> SETDDLKWTERLPECPVYRPTKEEFEDPLTYLQKIFPEASKYGICKIVSPLTATVPAGAVLMKEKSNFKFTTRVQPLRLAEWDSDDKVTFFMSGRTYTFRDYEKMANKVFARRYCSGGSLPDSFLEKEFWKEIACGKTETVEYACDVDGSAFSSAPGDPLGSSKWNLNKVSRLPKSTLRLLETSIPGVTEPMLYIGMLFSMFAWHVEDHYLYSINYQHCGASKTWYGIPGSAALKFEKVVKECVYNDDILSTNGEDGAFDVLLGKTTIFPPKTLLDHNVPVYKAVQKPGEFVVTFPRAYHAGFSHGFNCGEAVNFAMGDWFPFGAIASCRYAHLNRVPLLPHEELICKEAMLLNSSSKSENLDLTPTELSGQRSIKTAFVHLIRFLHLARWSLMKSGLCTGLVSNTYGTIVCSLCKRDCYLAFINCECYSHPVCLRHDVKKLDLPCGTTHTLYLRDNIEDMEAAAMKFEKEDGVSDLITTDEDLYKYPSS

Here we investigate the role of histone demethylases in plant flowering through the analysis of Arabidopsis JMJ13, which we show possesses H3K27me3 site-specific demethylase activity in vitro and in vivo. The recombinant expressed JMJ13 catalytic domain (JMJ13CD, residues 90–578) displayed unambiguous demethylation activity against H3K27me3 peptides, but not H3K4me3, H3K9me3, or H3K36me3 peptides, confirming that JMJ13 is an H3K27me3 site-specific histone demethylase. JMJ13 has a central catalytic domain flanked by flexible regions on both N- and C-termini. Our genetic studies suggest that JMJ13 acts as a flowering repressor, which modulates flowering time in a temperature- and photoperiod-dependent manner.

The crystal structure of the JMJ13 catalytic domain (JMJ13CD), including the predicted jumonji, helical, and zinc finger domains, in complex with the co-factor α-ketoglutarate (α-KG), was determined to 2.4 Å resolution. Despite being in different subfamilies, the overall structure of JMJ13CD resembles the previously reported structures of human KDM5A/B/C and Arabidopsis JMJ14, which are composed of two parts: the jumonji domain and the helical plus zinc finger domains. The jumonji domain adopts a typical α-KG-dependent oxygenase fold with a double-stranded β-helix in the center surrounded by several α-helices. A Ni2+ ion, which replaced the endogenous Fe2+ ion during nickel column purification, and the co-factor α-KG are located in the active center of the jumonji domain. The helical domain consists of four long α-helices forming a helical bundle. However, our structural analysis showed that the predicted C5HC2 zinc finger of JMJ13 in fact adopts a C4HCHC arrangement, which is composed of a CCCH-type zinc finger (Cys500, Cys503, Cys522, and His525) and a CCHC-type zinc finger (Cys514, Cys516, His519, and Cys534). Rather than the predicted Cys507, the His525 contributes to zinc coordination in the C4HCHC-type zinc finger domain in JMJ13. Although the C4HCHC zinc finger domain is embedded in the primary sequence of the helical domain, structurally it forms an independent domain that interacts with the helical domain in a similar manner to the helical and C5HC2 domains of JMJ1424.Single-stranded DNA-binding proteins (SSBs) play a crucial role in DNA metabolism by binding and stabilizing single-stranded DNA (ssDNA) intermediates. The majority of SSBs adopt homotetrameric configurations for activity. Diverging from E. coli, which harbors a solitary SSB variant (EcSSB), certain bacteria like Staphylococcus aureus exhibit a more complex scenario with the presence of three paralogous SSBs, specifically referred to as SaSsbA, SaSsbB, and SaSsbC. Of these, SaSsbA may be an EcSSB counterpart due to its possession of an acidic tip and sequence resemblance to EcSSBn.

The crystal structure of glycerol-bound SaSsbA was successfully determined at a resolution of 1.8 Å. While SaSsbA is typically active as tetramers, this glycerol-bound structure contained only two monomers of SaSsbA within each asymmetric unit. In contrast to the crystal structure of apo-SaSsbA, this structure displayed two additional amino acid residues, namely P105 and K106, as indicated by the blue mesh, solely in the subunit A of SaSsbA. In congruence with the apo form, the overall architecture of this glycerol-bound SaSsbA monomer remained characteristic of an OB-fold structure, marked by a β-barrel (composed of 5 β-strands) crowned with an α-helix. Within this structure of an SaSsbA dimer, two glycerol molecules (designated as Glycerol 1 and Glycerol 2) were present. However, these glycerol molecules exhibited distinct binding patterns to SaSsbA (see below). Among these interacting residues were F48 (Subunit B), N50 (Subunit B), S79 (Subunit A), R80 (Subunit A), F91 (Subunit A), V92 (Subunit A), and T93 (Subunit A). In light of the interactions identified through PLIP, it was established that the main chains of R80 and V92, along with the side chains of S79 and T93, partook in hydrogen bonding with Glycerol 1. Specifically, M1 (Subunit A), L2 (Subunit A), N3 (Subunit A), R4 (Subunit A), T36 (Subunit B), F37 (Subunit B), R76 (Subunit A), and D98 (Subunit A) were observed to participate within contact distance (<4 Å) in binding interactions with Glycerol 2. The structural evaluation conducted via PLIP underscored that the main chains of M1, N3, and T36, as well as the side chain of R76, were pivotal components in the hydrogen bonding network, fostering the binding of Glycerol 2.

>MLNRVVLVGRLTKDPEYRTTPSGVSVATFTLAVNRTFTNAQGEREADFINCVVFRRQADNVNNYLSKGSLAGVDGRLQSRNYENQEGRRVFVTEVVCDSVQFLEPKHHHHHH[2x]>MVMAGASSLDEIRQAQRADGPAG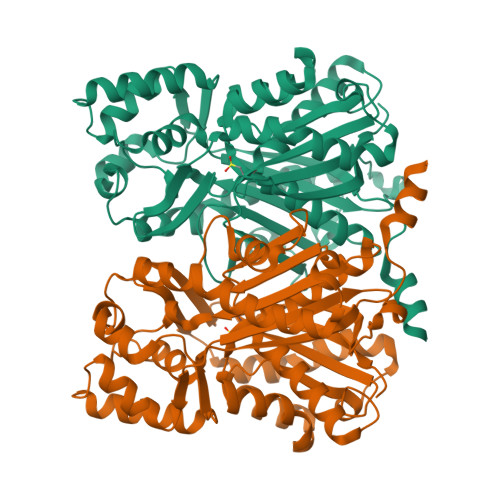ILAIGTANPENHVLQAEYPDYYFRITNSEHMTDLKEKFKRMCDKSTIRKRHMHLTEEFLKENPHMCAYMAPSLDTRQDIVVVEVPKLGKEAAVKAIKEWGQPKSKITHVVFCTTSGVDMPGADYQLTKLLGLRPSVKRLMMYQQGCFAGGTVLRIAKDLAENNRGARVLVVCSEITAVTFRGPSDTHLDSLVGQALFSDGAAALIVGSDPDTSVGEKPIFEMVSAAQTILPDSDGAIDGHLREVGLTFHLLKDVPGLISKNIVKSLDEAFKPLGISDWNSLFWIAHPGGPAILDQVEIKLGLKEEKMRATRHVLSEYGNMSSASVLFILDEMRRKSAKDGVATTGEGLEWGVLFGFGPGLTVETVVLHSVPL[4x]> GSSIN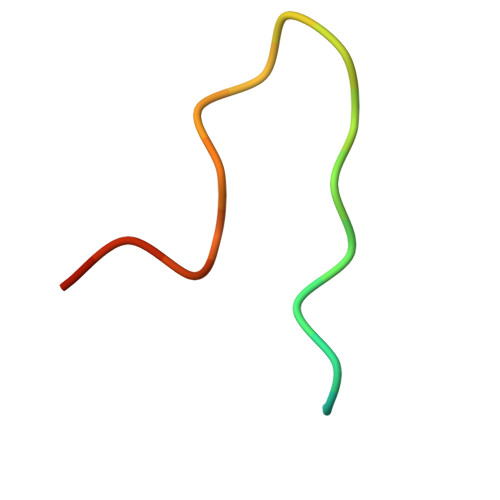WPPEFHPGVPWKGLQNI>GLKSTVESALTRRIMGIETEYGLTFVDGDSKKLRPDEIARRMFRPIVEKYSSSNIFIPNGSRLYLNVGSHPEYATAECDNLTQLINFEKAGDVIADRMAVDAEESLAKEDIAGQVYLFKNNVDSVGNSYGCHENYLVGRSMPLKALGKRLMPFLITRQLICGAGRIHHPNPLDKGESFPLGYCISQRSDHVWEGVSSATTRSRPIINTRDEPHADSHSYRRLHVIVGDANMAEPSIALKVGSTLLVLEMIEADFGLPSLELANDIASIREISRDATGSTLLSLKDGTTMTALQIQQVVFEHASKWLEQRPEPEFSGTSNTEMARVLDLWGRMLKAIESGDFSEVDTEIDWVIKKKLIDRFIQRGNLGLDDPKLAQVDLTYHDIRPGRGLFSVLQSRGMIKRWTTDEAILAAVDTAPDTTRAHLRGRILKAADTLGVPVTVDWMRHKVNRPEPQS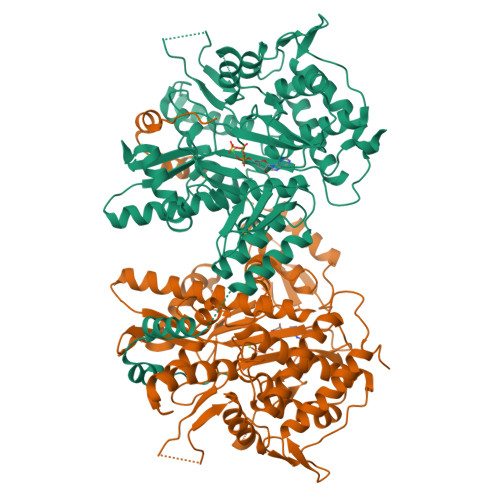VELGDPFSAVNSEVDQLIEYMTVHAESYRSGSASGTSLLDEIDGLLENNAEEFVRSYVQKGGE[2x]>[2x]PISPIETVPVKLKPGMDGPKVKQWPLTEEKIKALVEICTEMEKEGKISKIGPENPYNTPVFAIKKKDSTKWRKLVDFRELNKRTQDFWEVQLGIPHPAGLKKKKSVTVLDVGDAYFSVPLDEDFRKYTAFTIPSINNETPGIRYQYNVLPQGWKGSPAIFQSSMTKILEPFKKQNPDIVIYQYMDDLYVGSDLEIGQHRTKIEELRQHLLRWGLTTPDKKHQKEPPFLWMGYELHPDKWTVQPIVLPEKDSWTVNDIQKLVGKLNWASQIYPGIKVRQLSKLLRGTKALTEVIPLTEEAELELAENREILKEPVHGVYYDPSKDLIAEIQKQGQGQWTYQIYQEPFKNLKTGKYARMRGAHTNDVKQLTEAVQKITTESIVIWGK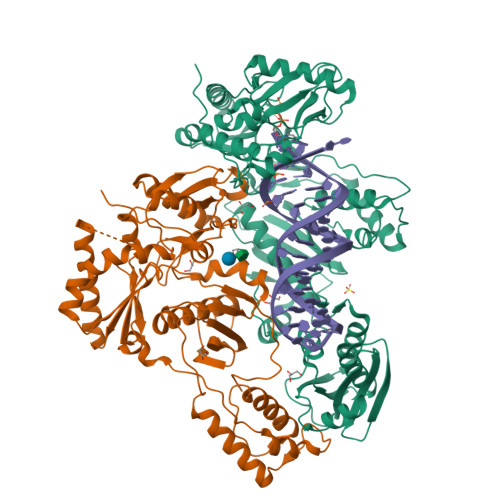TPKFKLPIQKETWETWWTEYWQATWIPEWEFVNTPPLVKLWYQLEKEPIVGAETFYVDGAANRETKLGKAGYVTNKGRQKVVPLTNTTNQKTELQAIYLALQDSGLEVNIVTNSQYALGIIQAQPDKSESELVNQIIEQLIKKEKVYLAWVPAHKGIGGNEQVDKLVSAG;>[2x]GPISPIETVPVKLKPGMDGPKVKQWPLTEEKIKALVEICTEMEKEGKISKIGPENPYNTPVFAIKKKDSTKWRKLVDFRELNKRTQDFWEVQLGIPHPAGLKKKKSVTVLDVGDAYFSVPLDEDFRKYTAFTIPSINNETPGIRYQYNVLPQGWKGSPAIFQSSMTKILEPFKKQNPDIVIYQYMDDLYVGSDLEIGQHRTKIEELRQHLLRWGLTTPDKKHQKEPPFLWMGYELHPDKWTVQPIVLPEKDSWTVNDIQKLVGKLNWASQIYPGIKVRQLSKLLRGTKALTEVIPLTEEAELELAENREILKEPVHGVYYDPSKDLIAEIQKQGQGQWTYQIYQEPFKNLKTGKYARMRGAHTNDVKQLTEAVQKITTESIVIWGKTPKFKLPIQKETWETWWTEYWQATWIPEWEFVNTPPLVKLWYQ> NMRVTQ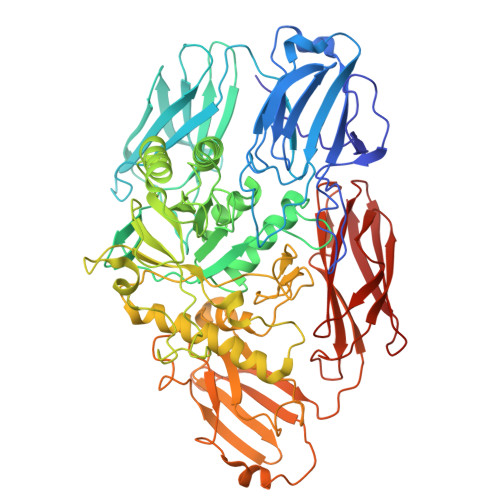KLNHGWIFAEGAADPATPLAGETVTLPHNAVDLPLSYFDETSYQRAFTYQRVIAWDDAWQGRRVQLRFDGAMADNVVWVNGVQVVAHPDGYTPFVADLTDHLRPGDNLVTVRIDGSENPAIPPFGAQIDYLTYAGIYRDVWLMVLPERHLTNARILTPDALSDAKTVVIRPEVTAPGPVRARLLDGDREIAATEGEGELTLAGLTGLSLWSTDNPQLYTVELTLPDSGDVTTHRFGFRTAEWTPQGFLLNGQPMKLRGLNRHQSWAHQGYAAGRHAQERDAEIVRHDLCCNMVRTSHYPQSTWFLDRCDEIGLLVFEEIPGWQHIGDQAWQDRSVDNVRAMITRDWNHPSIVIWGVRINESPDNHDFYVRTNALARELDPTRAIGGVRCITDSEMLEDVYTMNDFILDESELPLINRPRTALRPTEEVTGIKKPVPYLVTEYNGHMFPTKAQDPELRQMEHVIRHLEVLNAAHGDPAISGCIGWCMFDYNTHKDFGAGDRICHHGVMDIWREPKFAAHAYGSQKPPSEGIVMEPVTFWARGERNIGGVLPLIVLTNCDEVEFECAGVTRRVGPDRERFPHLPRPPVIIDHRHISAEELGQWGMSWHPGRITGWLNGEQVALREYVADPLPTTLQIAPDRDTLPADGDIDLRVMLRALDQVGNRLPFLDAGIAVTVDGPARLIGPDLRMLQGGTTGMLLRLTGDAGTIRITARHPQFPEAVATVTVG> GPQSEPELKLESVVIVSRHGVRAPTKATQLMQDVTPDAWPTWPVKLGWLTPRGGELIAYLGHYQRQRLVADGLLAKKGCPQSGQVAIIADVDERTRKTGEAFAAGLAPDCAITVHTQADTSSPDPLFNPLKTGVCQLDNANVTDAILSRAGGSIADFTGHRQTAFRELERVLNFPQSNLCLKREKQDESCSLTQALPSELKVSADNVSLTGAVSLASMLTEIFLLQQAQGMPEPGWGRITDSHQWNTLLSLHNAQFYLLQRTPEVARSRATPLLDLIKTALTPHPPQKQAYGVTLPTSVLFIAGHATNLANLGGALELNWTLPGQPDNTPPGGELVFERWRRLSDNSQWIQVSLVFQTL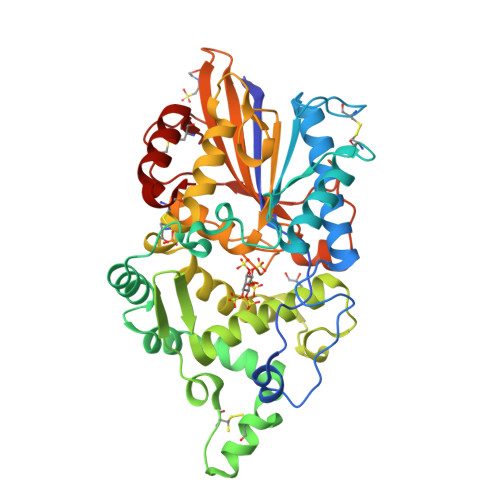QQMRDKTPLSLNTPPGEVKLTLAGCEERNAQGMCSLAGFTQIVNEARIPACSL NITROBENZENE | C6 H5 N O2 | 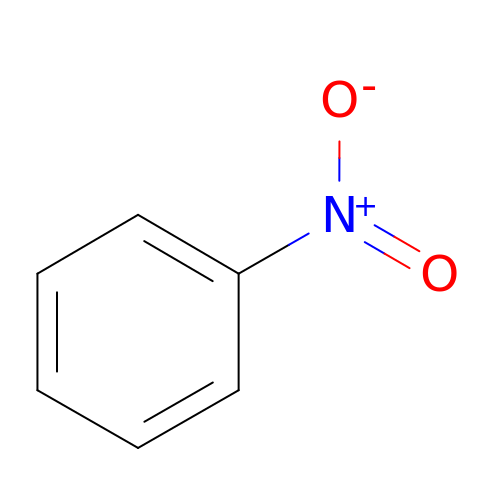LQNUZADURLCDLV-UHFFFAOYSA-N>[2x]MEKKKKLILFDFDSTLVN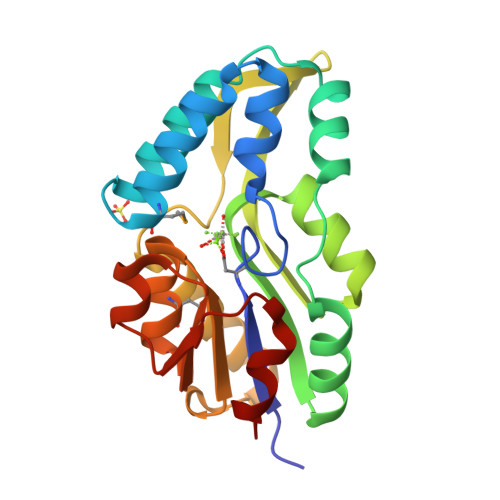NETIDEIAREAGVEEEVKKITKEAMEGKLNFEQSLRKRVSLLKDLPIEKVEKAIKRITPTEGAEETIKELKNRGYVVAVVSGGFDIAVNKIKEKLGLDYAFANRLIVKDGKLTGDVEGEVLKENAKGEILEKIAKIEGINLEDTVAVGDGANDISMFKKAGLKIAFCAKPILKEKADICIEKRDLREILKYIK> GSGSTRDYEIQRERIELGRCIGEGQFGDVHQGIYMSPENPALAVAIKTCKNCTSDSVREKFLQEALTMRQFDHPHIVKLIGVITENPVWIIMELCTLGELRSFLQVRKYSLDLASLILYAYQ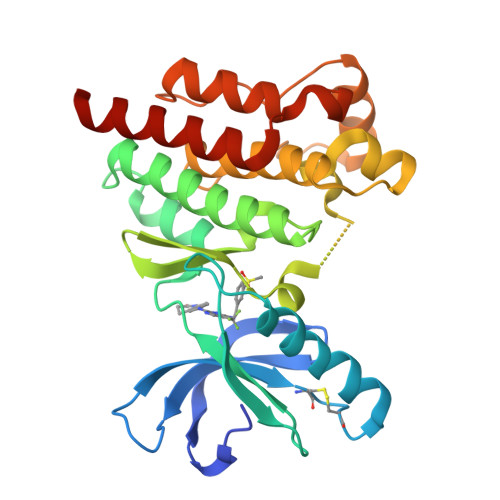LSTALAYLESKRFVHRDIAARNVLVSSNDCVKLGDFGLSRYMEDSTYYKASKGKLPIKWMAPESINFRRFTSASDVWMFGVCMWEILMHGVKPFQGVKNNDVIGRIENGERLPMPPNCPPTLYSLMTKCWAYDPSRRPRFTELKAQLSTILEEEKAQQEE>GHMWSATNEEDDLSVEAEIAHQIAESFEKKYKFPSRSSGIFLYNFEQLKMNLDDIVKEAKNVP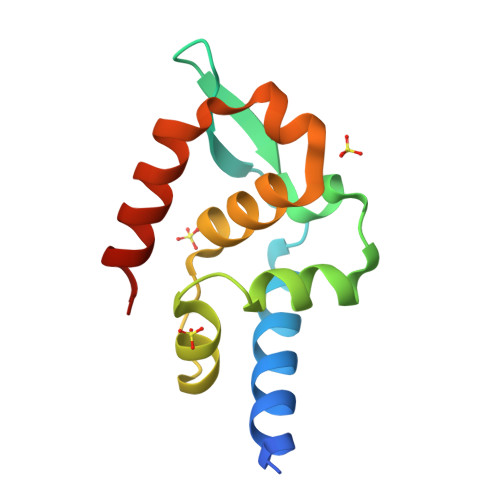GVTRLAHDGSKLPLRCVLGWVALANSKKFQLLVEANKLNKIMQDDLNRYASS[2x]> GGSMQAIKCVVVGDGAVGKTCLLISYTTNAFPGEYIPTVFDNYSANVMVDGSGLATTLERIEKNFVITDPRLPDNPIIFASDSFLQLTEYSREEILGRNARFLQGPETDRATVRKIRDAIDNQTEVTVQLINYTKSGKKFWNLFHLQPMRDQKGDVQYFIGVQLDGTEHVRDAAEREGVMLIKKTAENIDEAAKELGSGGKPVNLGLWDTAGLEDYDRLRPLSYPQTDVFLICFSLVSPASFENVRAKWYPEVRHHCPNTPIILVGTKLDLRDDKDTIEKLKEKKLTPITYPQGLAMAKEIGAVKYLECSALTQRGLKTVFDEAIR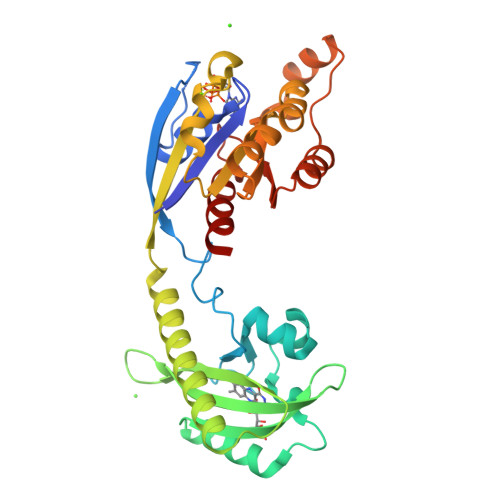AVLCPP>[2x]MTAVVKNLAKLPAATSQILTNVSKLQTFHGLLEERRDKYAPLAYHTYDNLKQKTTWHPIAHAWVDEGLPVSKKEYNEYCWLKKDMQRLLPLASPFVFGIYGILPLAVWLSNDGYLPSAFSSKKDIVSKKLEWYSSYGDDLRQQVGPMLQHRLKRHLRGTLNNEHRLMLDEVTESYKEIFYSHYTGQLRDVRKCAHLRLYDGTSTVLLLTNKEPVELTSELLQKWNAIKAAKLSPEEEKKARNEALIEAYKEQELHGGPHVKHMQGYGIPADTPLLGENAKGDQYTQPPESASIPLEQLEWTGDTVFIPAEYRTEMEDWGRELTKLANQFLLLPWRFVSNAWNQRRLVSWFEEILQEDALIAKEGGVQALSDDELKVALLDRAVIRCDEELTRGDMEARYKEISWLMSLRNPFIVLAWQTGYYRSTYSPEDDLPEASILPKLNRTVLDVDVHNELAPDHPEKPLPRVHPALYPNSHLALAKEVAVLAK;>[2x]MAAKTIPFVASTALGERLFAGVQKVLAAAKAPVSLVQTDAKFAPADAKYLLAEPLSAAATGELANKYGLSSKVTSGAASQFYPNSIYPSLNVEVVQNLYALSNPAFSSLSATTTKAVTVKDESAIKLAELQKETERNISSFFRDEANKSVQATLRLACDKAIKTKADKKTVMVVTKPHGDAFDDLLAQVTKSESDGRADELRNSSVSVEPTLVGNAWPKLVMFPEGVNVVVCGPNASGDQVAQLFVGIAGGTGMVAQQLVGDAVVFTSANAEDNENPTGALLAASNLLTALGHEAEAKKIAAAVAKAYTTDRILPKELPGGKADLEAFIDAVAKHASA;>MTHAELHLFDLDEFMQTYKRLQTRQDWLIENKCKKSRLFSYVAAVIAFTVGKSATMSDEAILAKIDPYVTSEVRVQRGAWWRSGYFTKEEVEMMTPKGPIARYYKFLLGVRRFPLKHGALSWACGFVPAWLTFTSLNHWAQNRRLNRYLTQESVFGEMARELVRGKTADEATTSVMARVEKEILGVH[2x];>[2x]MSSYTGAALAPKSERLRLAFEEKQKDHQKCIEEAKGKGLKKDELIDACAWTHRKTILALKDWFAYRPPFQD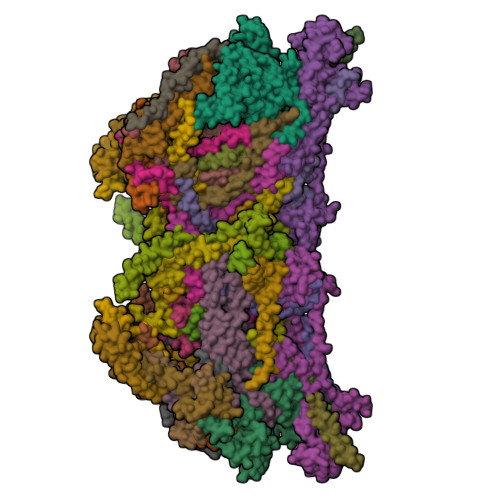RRSKWAEYCSIRHDSGSWLGWSQKFF;>[2x]MLNSNIYIIIYGGIIMYSIMIIIQMFLYNFSNKIYIEVEINKYILSKNNIDIYWIICNCTIIIIITTLNHIINKIGIYNMIEYNICYWLIGTGLGLYISPFIVFGYKFFVYIMDLNNYSLNIYHNNNKMNDIQQIYNGTNYNDTMIFFIKDINNIFTIYRSINFFMNWLYQMIYYGVRMWLVFVLHSFSLGSFGELITVITDNNLIFNVFYIGLLGLGFILYLIVIFYLGIQIYVYISFSLSFLHSTILLFLVNYIPHYNNKSIFNTFTNKSIY;>[2x]MPSTSPADKDVPMSILHTHGLSYVNWCMSLAPGLLVFEGFFRARYYRSRVPPSRTVLMNGLKMRMFSLARQQAPKIVHKPVLSPIPEHLRLVKNVAQVQIDMLKLLNAQAAK;>MMRRACRIIRPSHVRGVSGVAPTIYLRSKAALPATSTTDVRPQLYALQRFAKAQLKTATEAERAAIEADIARYQEYLDSDLEKLKQDVAEDTAKKQKLIPLLDRYPDVPIEKIPEHANVLLKKIDACLEILSKDIGEVTDAEAHEMYFETSKFQILHIYTGCVASFPEGDVPPGAVECLPGQVIRTKVNGEDVMLEIDEVDPGYQVCWFKPDVPLPENAEILWSYPYEPTAALPTGTTWEEGQANVLIPAEPTPEAAVWPPTPVTNVYAPMAEKLALKSNPELKVLFKEALLQPAKLLPLDVDYQCSHDREVVEAKRDRYLTALVEAEQAPPLPFTPDVLQLQLEHNVLKGELIDRLRALEYTIVTEQLQARLHERRLRGDVIDEWEELDYHPLVRDDTYLAIDFGDPTFGRYIWKLFPHTDGDEECMFKDTRLDVLPPQVNPLNAILAQHTAQTPVHRSLEKRLWTEVRATAVSE[2x];>[2x]MAPLYPVLSQASLYKRHFFKNIKLFHVVFYVGAPCVTFGTAAWSGSNRNSREAIFMVIEERHGWDNFKKLSSHQQGVIMQEAAQESLLARNKGELHLP;>[2x]MVYTNWQSSYTRLFVSKPWMWHPLAWMTLSVGIWWKFGKESLCNERSFYIHTHPKWAPHKFHTVYNWSRDPIKWTLAEQYASIIRNTNTDIEAVLKIKLPANAN;>[2x]MAFGRTRPTLSSPLVPVWNDLRALQVFTSQEYMQKRGPGFTNTLEYKLSCLNPVKWYDMMKVMPGGKAFVGTALGLALFGGWGVEFVKNISVMTKEKPPIDWNNEKLGHLTRS;>LIPVSLVDLININIIFYILLLYTLLLFFIPLFLASINYTYHYIYKYYNYNYNFINNN[2x];>MSLAKVWMYASWIPRGIPKAMANELSSAAAALAHPEAIARVAQLESQGKNPYRVARAEFWQMYLACWPYRFRNTVVEWETCKAKVLKGSVDLQDIVDLLYLLAWAYLFWILGEIYGRGSLYGYRFDGEIHRQEAQNVILYKEKEAQEMAVVMEKLEKEIQEWLKTMEQE[2x];>[2x]MPLPNAVVQGYTSVRGPKRPLDHFYGRTPLNIDTLWHWVKFPHRYDNLRFAVCFWAFLVSAHFANKKQRNLRVEWEKNMEIQKKLHPSGLWSEEQAFAAAEKLGRPKAGHPMRVFEDGYQQFDLKPKLFDPDEEAHH;>[2x]MADHNKKDVGSWASPNEHLMFFDFSSWLLVDFGKRWERWVSFKKSFLTTTRSPYWSPQFFLLTFFQLRNSNVKLCENWNWAPKGDDFNLLHNSAAEPFGRDLKAHLEREAGAKHHH;>[2x]MGGDAHAAPAEKPDPALDATKALPKALEEVEFFQSYAVRRKTGFHLFNRATGSPTIVGPMFYNLYNFVRIGRVSKYVCWLSLPLVFQRMWMKNRATGMEYDIDLENYAPFEAKKNPMHGH;>MSLPTFFLAPPLTEPFRARHRRKCIEKKDTFFQCLDKNKNETEPCEVEASGYSQECPDSWRRYFNEQRWKALELKGEVKHANLKNTQQHF[2x];>MFGVTRKLLGELSEYVEVNEKGMPKPQALSLWNMPYAKRRALTKFARGVRWQFIVLFIALYNFKNRDDSHLLRRGAYN[2x];>[2x]MMRISRKLLVPVANFRPKKPWDGPWGIQISQKKDRPFIAMWILFPLLLVDHLTREYYAYWHSSKVPVTDVFGDF;>[2x]MGGKASEAVTIAFRFPHRTTFLVKQNVGQKLNKGHQTFWQLVAGGWLFFLLINRTSFKPKLAAPKV>[2x]PMILGYWNVRGLTHPIRLLL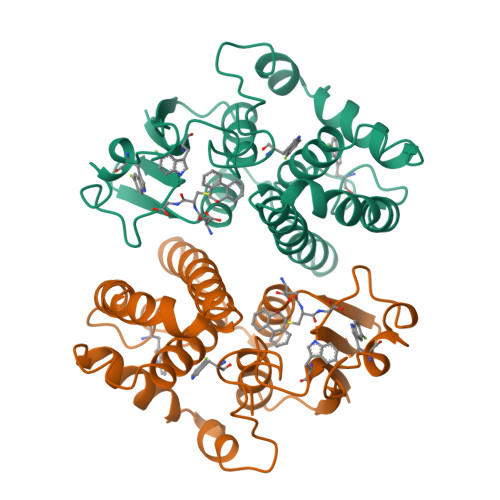EYTDSSYEEKRYAMGDAPDYDRSQWLNEKFKLGLDFPNLPYLIDGSRKITQSNAIMRYLARKHHLCGETEEERIRADIVENQVMDNRMQLIMLCYNPDFEKQKPEFLKTIPEKMKLYSEFLGKRPWFAGDKVTYVDFLAYDILDQYHIFEPKCLDAFPNLKDFLARFEGLKKISAYMKSSRYLSTPIFSKLAQWSNK>MKALTARQQEVFDLIRDHISQTGMPPTRAEIAQRLGFRSPNAAEEHLKALARKGVIEIVSGASRGIRLLQEEEEGLPLVGRVAAGEPLLAQQHIEGHYQVDPSLFKPNADFLLRVSGMAMKDIGIMDGDLLAVHKTQDVRNGQVVVARIDDEVTVKRLKKQGNKVELLPEN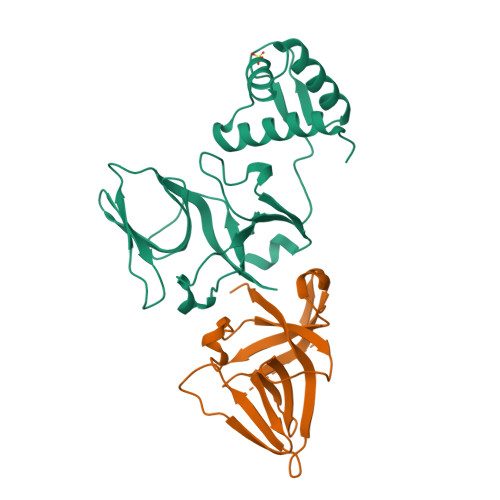SEFKPIVVDLRQQSFTIEGLAVGVIRNGDWL[2x]>[4x]MMVLRMKVEWYLDFVDLNYEPGRDELIVEYYFEPNGVSPEEAAGRIASESSIGTWTTLWKLPEMAKRSMAKVFYLEKHGEGYIAKIAYPLTLFEEGSLVQLFSAVAGNVFGMKALKNLRLLDFHPPYEYLRHFKGPQFGVQGIREFMGVKDRPLTATVPKPKMGWSVEEYAEIAYELWSGGIDLLKDDENFTSFPFNRFEERVRKLYRV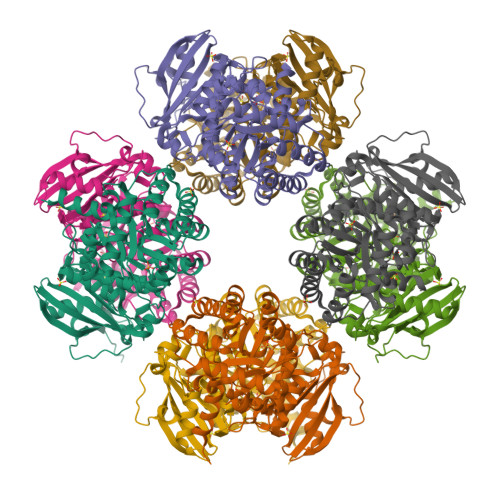RDRVEAETGETKEYLINITGPVNIMEKRAEMVANEGGQYVMIDIVVAGWSALQYMREVTEDLGLAIHAHRAMHAAFTRNPRHGITMLALAKAARMIGVDQIHTGTAVGKMAGNYEEIKRINDFLLSKWEHIRPVFPVASGGLHPGLMPELIRLFGKDLVIQAGGGVMGHPDGPRAGAKALRDAIDAAIEGVDLDEKAKSSPELKKSLREVGLSKAKVGVQH> IPEYVDWRQKGAVTPVKNQGSCGSCWAFSAVVTIEGIIKIRTGNLNQYSEQELLDCDRRSYGCNGGYPWSALQLVAQYGIHYRNTYPYEGVQRYCRSREKGPYAAKTDGVRQVQPYNQGALLYSIANQPVSVVLQAAGKDFQLYRGGIFVGPCGNKVDHAVAAVGYGPNYILIKNSWGTGWGENGYIRI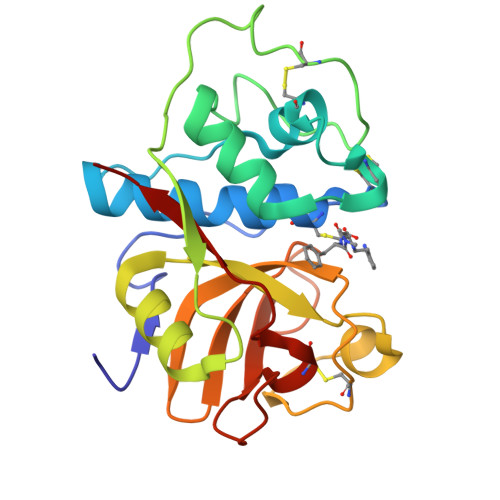KRGTGNSYGVCGLYTSSFYPVKN EBP catalyzes the conversion of Δ8-sterols (e.g zymosterol and zymostenol) to their corresponding Δ7-isomers. Here we present two structures of human EBP protein each in complex with a different pharmacologically active compound, revealing its mechanism of action in cholesterol biosynthesis and multidrug recognition. The structure was determined by selenium-based single-wavelength anomalous dispersion (SAD) and refined at 3.2 Å resolution with U18666A and 3.5 Å resolution with tamoxifen. This protein contains five transmembrane helices (TMs 1–5). EBP forms a homodimer in the crystal, as reported in previous solution studies, with dimensions of 65 × 30 × 55 Å.

However, when we supplemented the medium with either U18666A (an inhibitor of cholesterol biosynthesis and Niemann-Pick C1 protein)23,24 or tamoxifen, growth of the yeast was inhibited. Crystals were only obtained with U18666A or tamoxifen in space group P21212, owing to these two compounds presenting a high binding affinity to EBP. In the density map, the ligand (U18666A or tamoxifen) was determined unambiguously. Comparison between U18666A-bound and tamoxifen-bound structures revealed a similar conformation. We also showed that U18666A and tamoxifen bind to EBP in the same manner, implying the binding mode of EBP ligands. The compounds that bind to EBP have a positively-charged amine group, mimicking the carbocationic reaction sterol intermediate. Asn193 and Glu122 recognize the amine group of the ligand, which is stabilized through a π-cation interaction with Trp196. Trp196 is capable of stabilizing the compound through a π-cation interaction, while His76, Glu80, Glu122, and Asn193 may form electrostatic interactions and hydrogen bonds with the amine group, further enhancing the binding.

>MWSHPQFEKTTNAGPLHPYWPQHLRLDNFVPNDRPTWHILAGLFSVTGVLVVTTWLLSGRAAVVPLGTWRRLSLCWFAVCGFIHLVIEGWFVLYYEDLLGDQAFLSQLWKEYAKGDSRYILGDNFTVCMETITACLWGPLSLWVVIAFLRQHPLRFILQLVVSVGQIYGDVLYFLTEHRDGFQHGELGHPLYFWFYFVFMNALWLVLPGVLVLDAVKHLTHAQSTLDAKATKAKSKKN[3x]>MKLEPLLSDVPRLLMEADLVPVQGTRFQPTGFPDLGAAHYEGPDGRPMLLVESAQSMANRLETVCWDKDADDWVVPLRGLPVVKVLDKAGKPLTNSVLEAHRLNSPYILEGKDKTLFDLLKQELAHMEEGPVDIRKLAETLLKVDANAVLHGVFLAKKELAGGRLRLPRALSAFIEAEDVRVASSGGVKNDHVNPSGDTSRGFGNVPFARDEYVSPRIKAYFNLDLAQIRAFGLGEQVDRLLIALALYKVRRFLVHGLRLRTACDLDCQALRVTRPEGWEVPELSELEAALPGLIEAVAGEGRFAQPAVTIVTYEK[7x]

Here, we report the composition, structure and function of the type I-G Cascade CRISPR effector from Thioalkalivibrio sulfidiphilus, revealing key new molecular details. The unique Csb2 subunit processes pre-crRNA, remaining bound to the 3′ end of the mature crRNA, and seven Cas7 subunits form the backbone of the effector. Cas3 associates stably with the effector complex via the Cas8g subunit and is important for target DNA recognition. Structural analysis by cryo-Electron Microscopy reveals a strikingly curved backbone conformation with Cas8g spanning the belly of the structure.

For this, the size-exclusion-purified assembled complex containing Cas7, Cas8g and Csb2 in the presence of a 72 nt crRNA was used for the structure determination. Seven interlocking Cas7 subunits which form a crescent shaped structure bound to 42 nt of the crRNA that threads through the interlocking Cas7 subunits were clearly visualised in the CryoEM density. We built the individual Cas7 subunits using the AF2 predicted structure as a starting model. The Cas7 protein adopted the typical central RAMP (Repeat Associated Mysterious Protein) domain with extended β-hairpin region. As observed for other type I complexes, each of the Cas7 subunits occupies 6 nucleotides of the crRNA with a recurring periodic pattern of 5 + 1 nt, with the sixth base flipped out in the opposite direction to the remaining five. A beta hairpin emanating from the adjacent Cas7 subunit is positioned along the phosphate backbone of the sixth base, generating the kink. This structural arrangement creates an unpairing of crRNA and a target DNA at these sites. We can also trace the 5′-handle of the crRNA, which loops back and is not bound by the Cas7.1 subunit. In our CryoEM reconstruction, we did not observe discernible density near the 3′ end of the RNA corresponding to the Csb2 subunit. With seven Cas7 backbone subunits, the type I-G effector shows pronounced curvature of the crRNA, reminiscent of that seen for type I-F systems.> MATEIR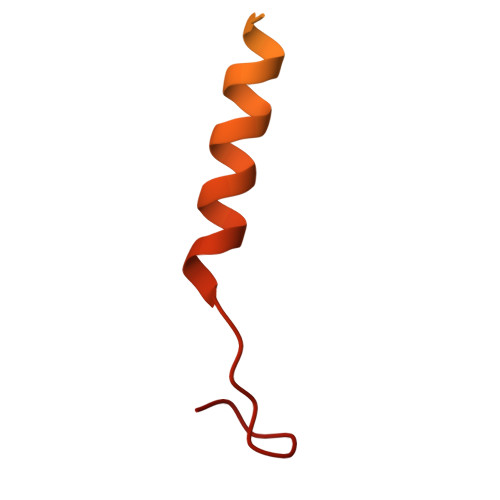VLKNVDDTVFYPKTHVTAVEGLDSATTTTSGLMPASDKTKLNGIEANAEKNNVTAIDIANWNKKQDAILVSENGSNFKITVTNAGELKATKVE> HHHHHHGSGTNVNDKVTASNFKLEKTTFDPNQSGNTFMAANFTVTDKVKSGDYFTAKLPDSLTGNGDVDYSNSNNTMPIADIKSTNGDVVAKATYDILTKTYTFVFTDYVNNKENINGQFSLPLFTDRAKAPKSGTYDANINIADEMFNNKITYNYSSPIAGIDKPNGANISSQIIGVDTASGQNTYKQTVFVNPKQR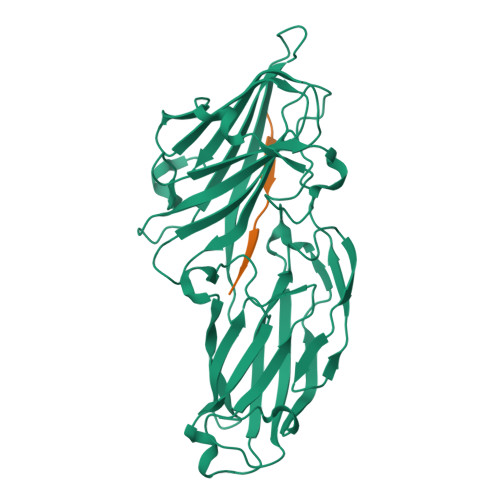VLGNTWVYIKGYQDKIEESSGKVSATDTKLRIFEVNDTSKLSESYYADPNDSNLKEVTDQFKNRIYYEHPNVASIKFGDITKTYVVLVEGHYDNTGKNLKTQVIQENVDPVTNRDYSIFGWNNENVVRYG;> YGGGSSGGGSSGGGH> EAQPAPHQWQKMPFWQKVRP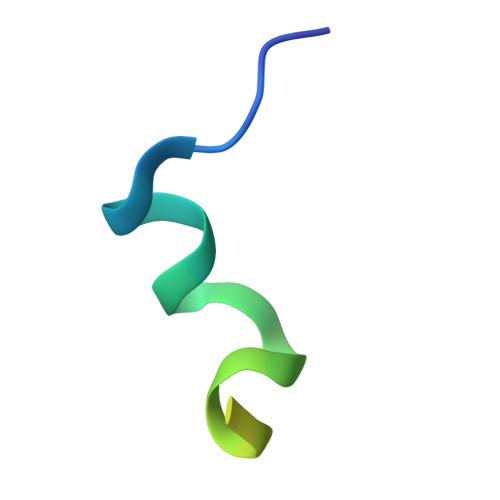WAAQLTQMGVAA>[2x]KNFLNIEELKRFLNGQTVVS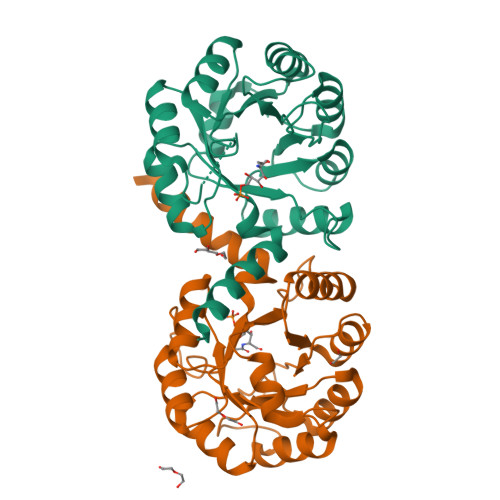IQPVTGSPLDKTDFIVAMAIAVEQAGAKALRIEGVSNVAAVSAAVTIPIIGIVKRDLPDSPVRITPFVSDVDGLANAGATVIAFDATNRTRPESRERIAQAIKNTGCFAMADCSTFEDGLWANSQGVEIVGSTLSGYVGDIEPTVPDFQLVKAFSEAGFFTMAEGRYNTPELAAKAIESGAVAVTVGSALTRLEVVTQWFNNATQAAGER> MGKTYDVNICYA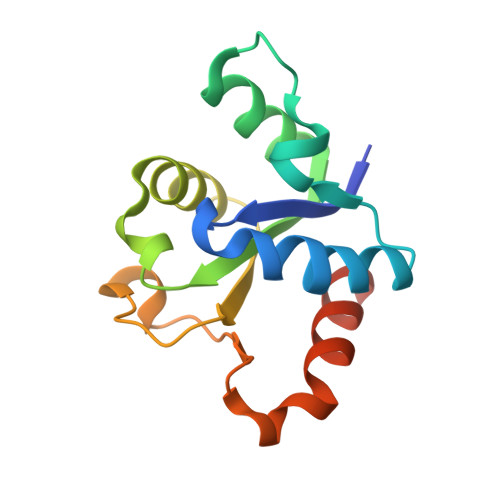PEDREWVINTLVFKLERAGIKTFVNIRDDTPGNFFAENIMDAIENSNRTIVVMSPDFFKNNICDKTLQIGLSHQIIPILYRPCEVPYFLNHMTYLDWCDKDVRPVFWRNLFRDIRNNHHHHHH>MTINATVKEAGFQPASRISSIGVSEILKIGARAAAMKREGKPVIILGAGEPDFDTPEHVKQAASDAIHRGETKYTALDGTPELKKAIREKFQRENGLAYELDEITVATGAKQILFNAMMASLDPGDEVIIPTPYWTSYSDIVHICEGKPVLIACDASSGFRLTAEKLEAAITPRTRWVLLNSPSNPSGAAYSAADYRPLLEVLLRHPHVWLLVDDMYEHIVYDGFRFVTPAQLEPGLKNRTLTVNGVSKAYAMTGWRIGYAGGPRELIKAMAVVQSQATSCPSSI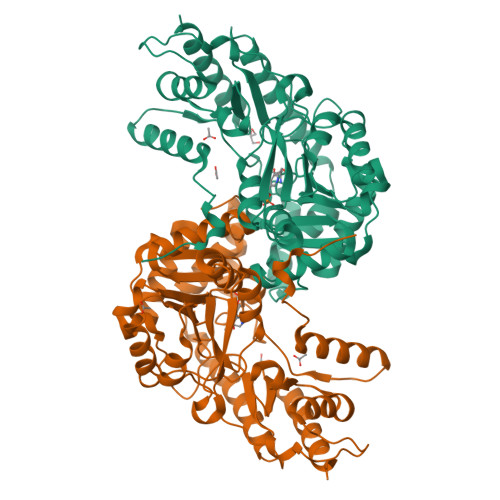SQAASVVALNGPQDFLKERTESFQRRRDLVVNGLNAIDGLDCRVPEGAFYTFSGCAGVLGKVTPSGKRIKTDTDFCAYLLEDAHVAVVPGSAFGLSPFFRISYATSEAELKEALERIAAACDRLS[2x]> GSHMTDRTDADD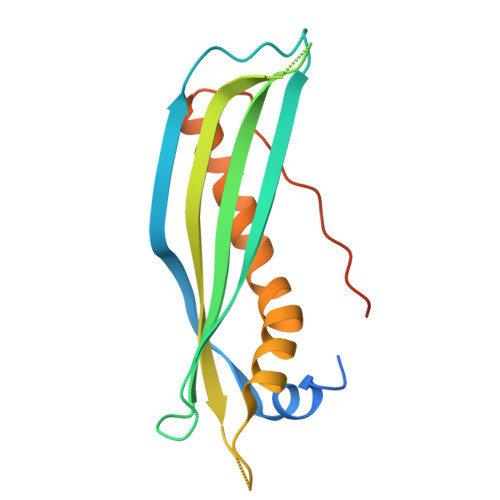LDLQRVGARLAARAQIRDIRLLRTQAAVHRAPKPAQGLTYDLEFEPAVDADPATISAFVVRISCHLRIQNQAADDDVKEGDTKDETQDVATADFEFAALFDYHLQEGEDDPTEEELTAYAATTGRFALYPYIREYVYDLTGRLALPPLTLEILSRPMPVSPGAQWPATRGTP>[9x]MAQILPIRFQEHLQLQNLGINPANIGFSTLTMESDKFICIREKVGEQAQVVIIDMNDPSNPIRRPISADSAIMNPASKVIALKAGKTLQIFNIEMKSKMKAHTMTDDVTFWKWISLNTVALVTDNAVYHWSMEGESQPVKMFDRHSSLAGCQIINYRTDAKQKWLLLTGISAQQNRVVGAMQ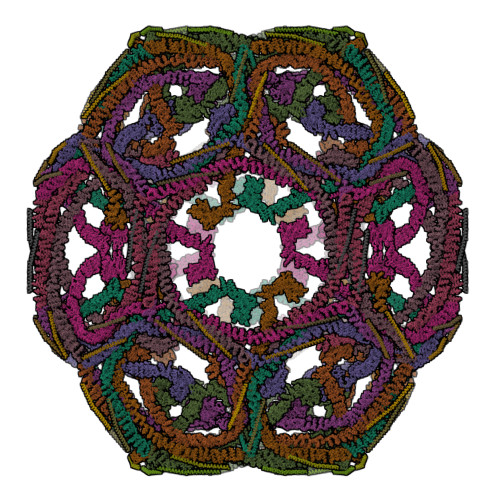LYSVDRKVSQPIEGHAASFAQFKMEGNAEESTLFCFAVRGQAGGKLHIIEVGTPPTGNQPFPKKAVDVFFPPEAQNDFPVAMQISEKHDVVFLITKYGYIHLYDLETGTCIYMNRISGETIFVTAPHEATAGIIGVNRKGQVLSVCVEEENIIPYITNVLQNPDLALRMAVRNNLAGAEELFARKFNALFAQGNYSEAAKVAANAPKGILRTPDTIRRFQSVPAQPGQTSPLLQYFGILLDQGQLNKYESLELCRPVLQQGRKQLLEKWLKEDKLECSEELGDLVKSVDPTLALSVYLRANVPNKVIQCFAETGQVQKIVLYAKKVGYTPDWIFLLRNVMRISPDQGQQFAQMLVQDEEPLADITQIVDVFMEYNLIQQCTAFLLDALKNNRPSEGPLQTRLLEMNLMHAPQVADAILGNQMFTHYDRAHIAQLCEKAGLLQRALEHFTDLYDIKRAVVHTHLLNPEWLVNYFGSLSVEDSLECLRAMLSANIRQNLQICVQVASKYHEQLSTQSLIELFESFKSFEGLFYFLGSIVNFSQDPDVHFKYIQAACKTGQIKEVERICRESNCYDPERVKNFLKEAKLTDQLPLIIVCDRFDFVHDLVLYLYRNNLQKYIEIYVQKVNPSRLPVVIGGLLDVDCSEDVIKNLILVVRGQFSTDELVAEVEKRNRLKLLLPWLEARIHEGCEEPATHNALAKIYIDSNNNPERFLRENPYYDSRVVGKYCEKRDPHLACVAYERGQCDLELINVCNENSLFKSLSRYLVRRKDPELWGSVLLESNPYRRPLIDQVVQTALSETQDPEEVSVTVKAFMTADLPNELIELLEKIVLDNSVFSEHRNLQNLLILTAIKADRTRVMEYINRLDNYDAPDIANIAISNELFEEAFAIFRKFDVNTSAVQVLIEHIGNLDRAYEFAERCNEPAVWSQLAKAQLQKGMVKEAIDSYIKADDPSSYMEVVQAANTSGNWEELVKYLQMARKKARESYVETELIFALAKTNRLAELEEFINGPNNAHIQQVGDRCYDEKMYDAAKLLYNNVSNFGRLASTLVHLGEYQAAVDGARKANSTRTWKEVCFACVDGKEFRLAQMCGLHIVVHADELEELINYYQDRGYFEELITMLEAALGLERAHMGMFTELAILYSKFKPQKMREHLELFWSRVNIPKVLRAAEQAHLWAELVFLYDKYEEYDNAIITMMNHPTDAWKEGQFKDIITKVANVELYYRAIQFYLEFKPLLLNDLLMVLSPRLDHTRAVNYFSKVKQLPLVKPYLRSVQNHNNKSVNESLNNLFITEEDYQALRTSIDAYDNFDNISLAQRLEKHELIEFRRIAAYLFKGNNRWKQSVELCKKDSLYKDAMQYASESKDTELAEELLQWFLQEEKRECFGACLFTCYDLLRPDVVLETAWRHNIMDFAMPYFIQVMKEYLTKVDKLDASESLRKEEEQATETQ;>VDRLQSEPESIRKWREEQTERLEALDANSRKQEAEWKEKAIKELDEWYARQDEQLQKTKANNRVADEAFY[9x]> GCCCGGAUAGCUCAGUCGGUAGAGCAG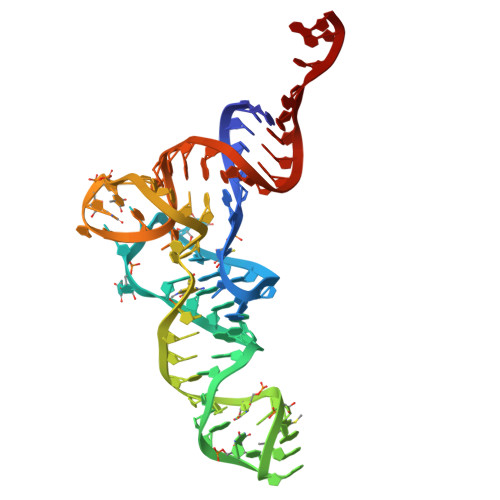GGGAUUGAAAAUCCCCGUGUCCUUGGUUCGAUUCCGAGUCCGGGCACCA(4~{S})-5-[4-[diethyl-[4-(2-ethyl-2-oxidanyl-butoxy)-3-methyl-phenyl]silyl]-2-methyl-phenoxy]-4-oxidanyl-pentanoic 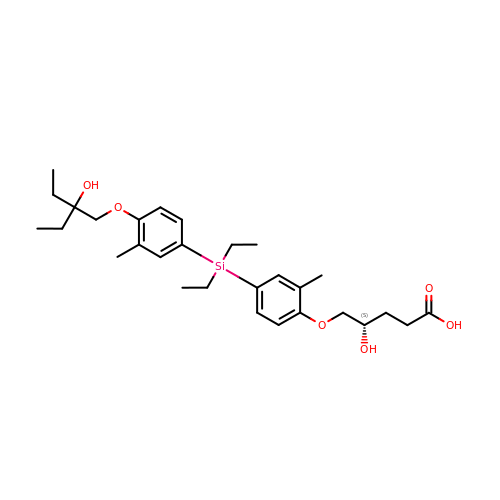acid | C29 H44 O6 Si | ACMSFXPVKXNDEF-HSZRJFAPSA-N>MGSDKIHHHHHHEEMEKGFDPKRYARELWFKLQDMMNEGLGYDAVEVLNTLDENPELAHQKFAKVVGVSNYRYYIIQGVGEIVEIKDDGILVKVRENRKVPDLFLSNHIFGNGIVNATGIAKMEDFDRIIDFNLTATE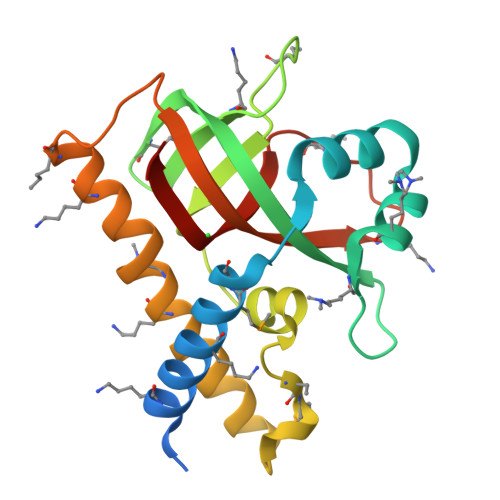LNKIVKEEVVNSFLKQLSKGAGSVGSLVRFIAVFTLLKDEEIKYPIEAIPLYLEIQGGF[4x]> MGHHHHHHMMKTKLPILGVLGGMGPVVTAEFLKSIYEYNPFIDKEQESPNVIVFSFPSAPDRTGSIDSGKEREFIDFIQVNLEHLNKLADCIVIGCCTAHYALPQIPENLKDKLISLIKIADQELQEYNEPTLLLASTGTYQKKLFQEGCTTADLIISLS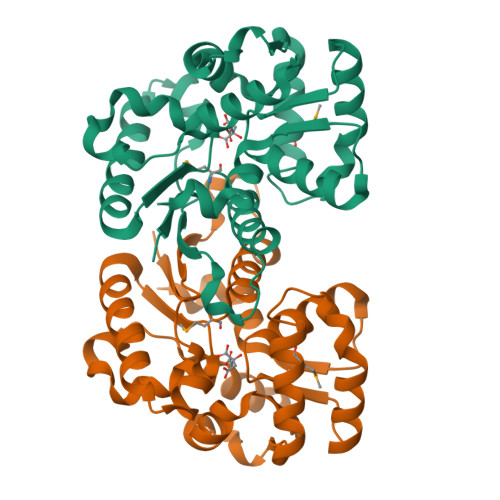ESDQKLIHEMIYKVLKRGHDPLSILRDIEALLEKYNTRSYISGCTEFHLLTKSLKLKGIDSIKAIDPLSTIAQNFSQLIIKQAQVDLVTDCHQPSNPKSP6-[(8E)-8-(1,3-benzothiazol-2-ylhydrazinylidene)-6,7-dihydro-5H-naphthalen-2-yl]pyridine-2-carboxylic acid | C23 H18 N4 O2 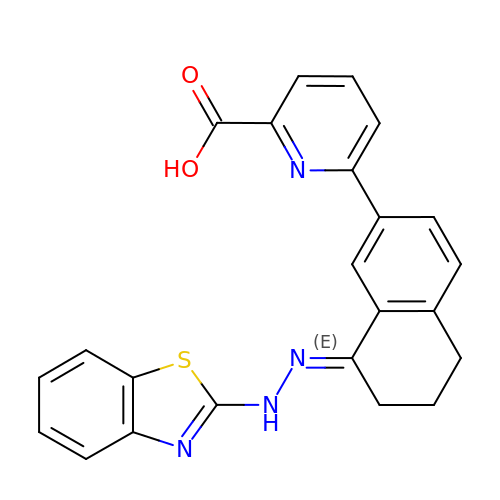S | ZGERKAMDOWOUTN-NLRVBDNBSA-N> GMKTQITTRDLVLEFIHALNTENFPAAKKRLNENFTFNGPMGHREGSERYMNDMEKMKFKYVVHKMFEEGNDVCLI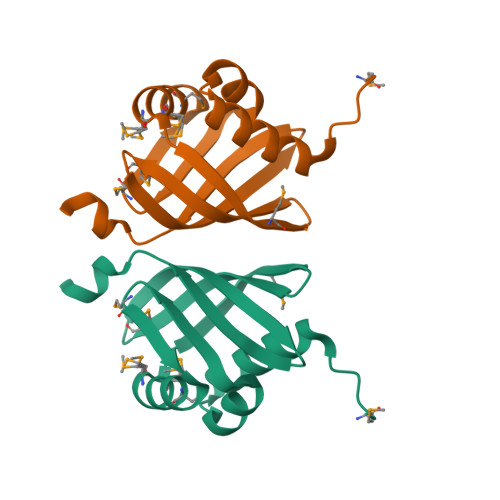YDINMNGKTIAASGLYHLEKGEITSLHVYFDPRPLFEE> GAMGSGIQRPRDKPLVFFNRQPSDPLTGKVDMAAMNWNDKTYYVGFDAKFGGSIQGKMILDFLASSESSVDRNGDGIIGYVLCIGDVGHNDSKVRTEGIR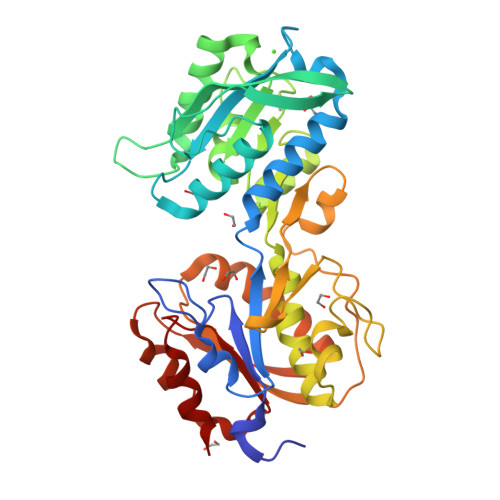RALGTWTGSSDPGQAKEGQAVVGGKSYKVVELEGKAMTGTDGSTANTNSATESMGSWVAKFADKIDLVISNNDGMAMGCLQASNYPRGLPIFGYDANADAVESVGKGELTGTVSQNVDAQAVAVLQIIRNLLDGSSGEDVVANGISRPDAHGNKISAPVQYWEDVKAIMADNSEVTSANWKEYTRGARDAGVRQVSAPTKKVLLTVHNASNDFLASAYLPALKHYAPLLNVDLTVVQGDGQNELSCLDKFTNLDMFDAFAVNMVKTNSGADYTDKLKY>MHHHHHHSSGRENLYFQGIKNVHVPDNYIIKHLIGRGSYGYVYLAYDKNTEKNVAIKKVNRMFEDLIDCKRILREITILNRLKSDYIIRLYDLIIPDDLLKFDELYIVLEIADSDLKKLFKTPIFLTEEHIKTILYNLLLGENFIHESGIIHRDLKPANCLLNQDCSVKVCDFGLARTINSEKDTNIVNDLEENEEPGPHNKNLKKQLTSHVVTRWYRAPELILLQENYTKSIDIWSTGCIFAELLNMLQSHINDPTNRFPLFPGSSCFPLSPDRNSKKVHEKSNRDQLNIIFNIIGTPTEDDLKNINKPEVIKYIKLFPHRKPINLKQKYPSISDDGINLLESMLKFNPNKRITIDQALDHPYLKD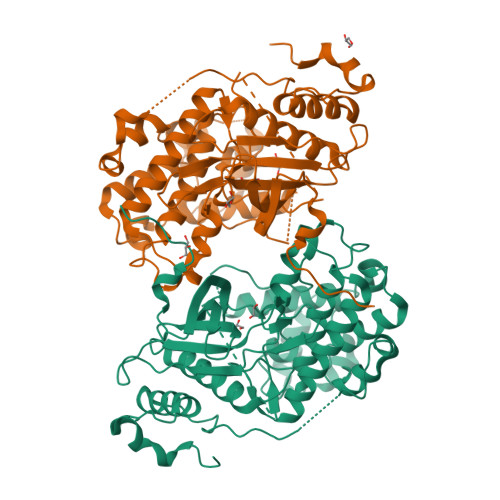VRKKKLENFSTKKIILPFDDWMVLSETQLRYIFLKEVQSFHPELVIPSVFTIHENNFYNNEKPSS[2x]> DDFAYL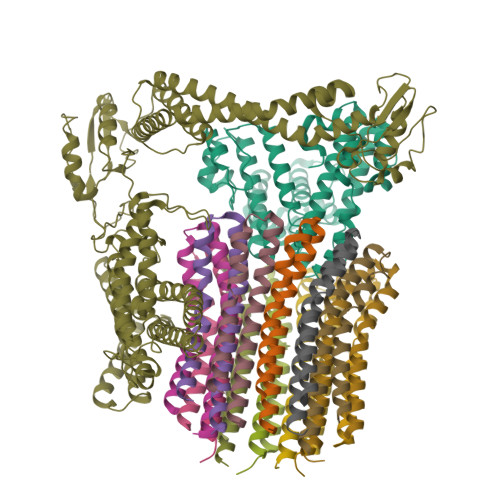NARVRVRRGTLLKESFFQEALDLSFADFLRLLSETVYGGELAGQGLPDVDRAVLRTQAKLVGDLPRLVTGEAREAVRLLLLRNDLHNLQALLRAKATGRPFEEVLLLPGTLREEVWRQAYEAQDPAGMAQVLAVPGHPLARALRAVLRETQDLARVEALLAKRFFEDVAKAAKGLDQPALRDYLALEVDAENLRTAFKLQGSGLAPDAFFLKGGRFVDRVRFARLMEGDYAVLDELSGTPFSGLSGVRDLKALERGLRCVLLKEAKKGVQDPLGVGLVLAYVKEREWEAVRLRLLARRAYFGLPRAQVEEEVVC;> MIAPMEKLVLAGPKGRAKELLQSLQQAGVVHLETLRPEALSAYQLSPEERAELRRWEAVSAGAEHTLSLLGLEAEPARPFPEGLEAAEKALSPIQAHAEGLTRQKQELEEELALAQAYLEPLERLAALAHGLDKSPFLRVIPFLLTEKELPLVEEALRKALEDRYLLAHEAYAGGVAALVVVHRKEVDQAKAALSRAGVAELRLPGALGELPLSEAARRLKERAEAAPRELSEVRQHLAKLARESASTLQSLWTRAQDEVARLKALEELASGRFGFALLGYVPVKAKPKVEEALARHKESVVYAFEPVDEHHEADRIPVVLDNPPWAKPFELLVSFLNTPKYGTFDPTPVVPVFFPFWFGMIVGDIGYALLFYLVGRWLSGYVKRNEPLVIDLFALKLKPQVIGKLVHILNWMVFWTVVWGVIYGEFFGTFLEHLGVFGTPEHPGLIPILIHRIDTAKTANLLILLSVAFGVVLVFFGLALRAYLGLKHRHMAHFWEGVGYLGGLVGVLALAASYLGNLQAGWLQGLMYLGFGVFLLAVLMSRIWLMIPEIFTQAGHILSHIRIYAVGAAGGILAGLLTDVGFALAERLGLLGVLLGLLVAGVLHLLILLLTTLGHMLQPIRLLWVEFFTKFGFYEENGRPYRPFKSVR;>[12x]GGLDRGLIAVGMGLAVGLAALGTGVAQARIGAAGVGAIAEDRSNFGTALIFLLLPETLVIFGLLIAFILNGRL Gas vesicles are gas-filled nanocompartments that allow a diverse group of bacteria and archaea to control their buoyancy. GVs have therefore evolved as rigid, thin-walled structures composed of a single protein unit that typically polymerizes into large cylindrical shells closed off by conical tips. The ∼7 kDa primary GV protein GvpA forms the core of the GV shell and the cone-shaped tips. Here, we report the 3.2 Å cryo-EM structure of the gas vesicle shell made from the structural protein GvpA that self-assembles into hollow helical cylinders closed off by cone-shaped tips.

We expressed and purified Bacillus megaterium GVs that form narrow tubes most suitable for cryo-EM analysis. We used a combination of two- and three-dimensional (2D and 3D) classification techniques to select 4% of the small GV subset corresponding to 35.6 nm diameter and used helical reconstruction to obtain a cryo-EM density of 3.2 Å resolution. The cylindrical shell is constructed from thousands of GvpA2 monomers polymerized side by side into ribs spiraling into a left-handed helix with a helical pitch of 48.8 Å and −3.87° helical twist, resulting in 92.93 GvpA2 units per helical turn. Contrary to postulated models, GvpA monomers and not antiparallel dimers form the repeating units of the helical assembly. The carboxyl-terminal residues Asp67-Ile88 are flexible and not resolved in our structure. The central β-hairpin, tilted at −36° relative to the long axis of the cylinder, forms the core of the GV ribs. Helix α2 folds back onto the hairpin, and helix α1 forms a bridge across the ∼16 Å gap separating adjacent ribs. The inner wall of the GV shell forms a continuous hydrophobic surface consisting of a dense pattern of hydrophobic residues located on the luminal side of the β-hairpin and helix α1. We located pores in the GV shell formed by slit-like openings between α1 helices of adjacent GpvA2 monomers. GvpA2 monomers are held together tightly by lateral connections along the GV ribs formed by an extensive hydrogen-bonding network between the β strand backbones.

> MSIQKSTNSSSLAEVIDRILDKGIVIDAFARVSVVGIEILTIEARVVIASVDTWLRYAEAVGLLRDDVEENGLPERSNSSEGQPRFSI> SNANDIRSKKVLIIGAGSLGSMIAENLMRIGVVSQGILDADLLQTGNL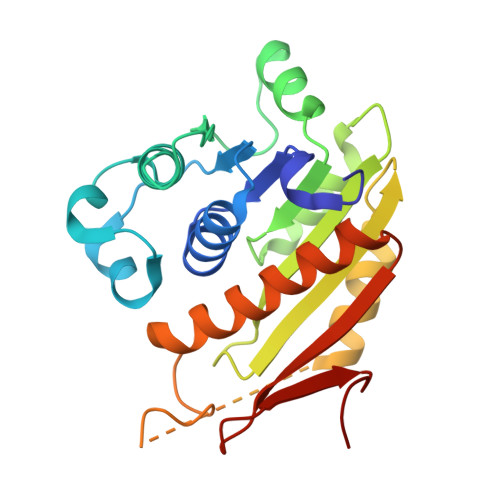SRHALTMTSVGHNKAAALVEHLNRILPDASARSFSCAFPPESEVAKNSLRQYDVIIDCTGDDGVLKSLAAFDWKSEKIFISLAMTWRAEGLFAFAASETSFPVTDASSRFNASASPEIDMDEARIEGIGAWHPVFPARADDVQLWAAVGTKFICRVVSAPGRIYEYFKQMPDGTVEKEPHEYGSG> GPLVPESLQEQIQSNFIIVIHPGSTTLRIGRATDTLPASIPHVIARRHKQQGQPLYKDSWLLREGLNKPESNEQRQNGLKMVDQAIWSKKMSNGTRRIPVSPEQARSYNKQMRPAILDHCSGNKWTNTSHHPEYLVGEEALYVNPLDCYNIHWPIRRGQLNIHPGPGGSLTAVLADIEVIWSHAIQKYLEIPLKDLKYYRCILLIPDIYNKQHVKELVNMILMKMGFSGIVVHQESVCATYGSGLSSTCIVDVGDQKTSVCCVEDGVSHRNTRLCLAYGGSDVSRCFYWLMQRAGFPYRECQLTNKMDCLLLQHLKETFC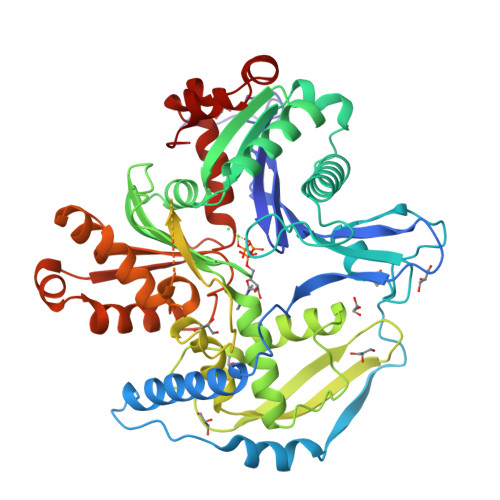HLDQDISGLQDHEFQIRHPDSPALLYQFRLGDEKLQAPMALFYPATFGIVGQKMTTLQHRSQGDPEDPHDEHYLLATQSKQEQSAKATADRKSASKPIGFEGDLRGQSSDLPERLHSQEVDLGSAQGDGLMAGNDSEEALTALMSRKTAISLFEGKALGLDKAILHSIDCCSSDDTKKKMYSSILVVGGGLMFHKAQEFLQHRILNKMPPSFRRIIENVDVITRPKDMDPRLIAWKGGAVLACLDTTQELWIYQREWQRFGVRMLRERAAFVW> IIGGTECRPHARPYMAYLEIVTPENHLSACSGFLIRRNFVMTAA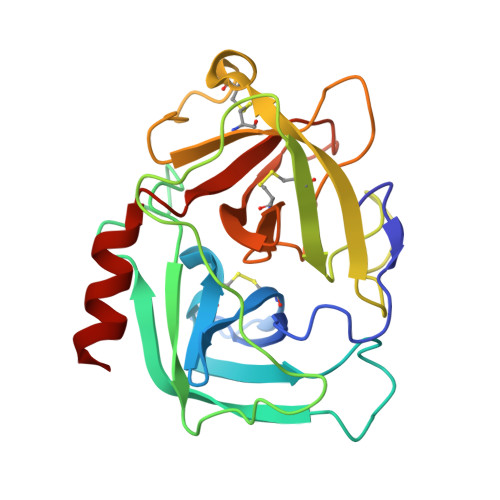HCAGRSITVLLGAHNKKVKEDTWQKLEVEKQFPHPKYDDRLVLNDIMLLKLKEKANLTLGVGTLPISAKSNSIPPGRVCRAVGWGRTNVNEPPSDTLQEVKMRILDPQACKHFEDFHQEPQLCVGNPKKIRNVYKGDSGGPLLCAGIAQGIASYVLRNAKPPSVFTRISHYRPWINKILREN> GAMGQSTSNHLWLLSDILGQGATANVFRGRHKKTGDLFAIKVFNNISFLRPVDVQMREFEVLKKLNHKNIVKLFAIEEETTTRHKVLIMEFCPCGSLYTVLEEPSNAYGLPESEFLIVLRDVVGGMNHLRENGIVHRDIKPGNIMRVIGEDGQSVYKLTDFGAARELEDDEQFVALYGTEEYLHPDMYERAVLRKDHQKKYGATVDLWSIGVTFYHAATGSLPFRPFEGPRRNKEVMYKIITGKPSGAISGVQKAENGPIDWSGDMPVSCSLSRGLQVLLTPVLANILEADQEKCWGFDQFFAETSDILHRMVIHVFSLQQMTAHKIYIHSYNTATIFHELVYKQTKIISSNQELIYEGRRLVLEPGRLAQHFPKTTEENPIFVVSREPLNTIGLIYEKISLPKVHPRYDLDGDASMAKAITGVVCYACRIASTLLLYQELMRKGIRWLIELIKDDYNETVHKKTEVVITLDFCIRNIEKTVKVYEKLMKINLEAAELGEISDIHTKLLRLSSSQGTIETSLQDIDSRLSPGGSLADAWAHQEGTHPKDRNVEKLQVLLNCMTEIYYQFKKDKAERRLAYNEEQIHKFDKQKLYYHATKAMTHFTDECVKKYEAFLNKSEEWIRKMLHLRKQLLSLTNQCFDIEE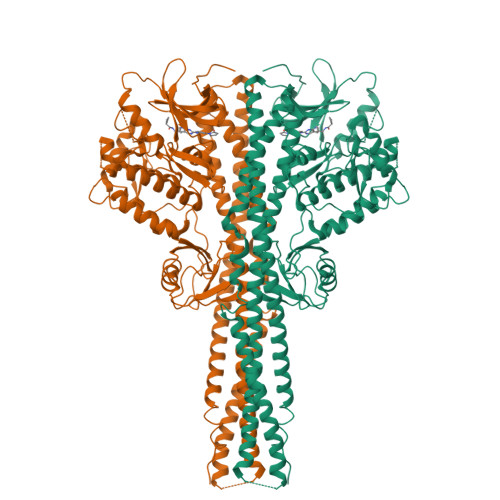EVSKYQEYTNELQET>GSMTEIALIGNPNSGKTSLFNLITGHNQRVGNWPGVTVERKSGLVKKNKDLE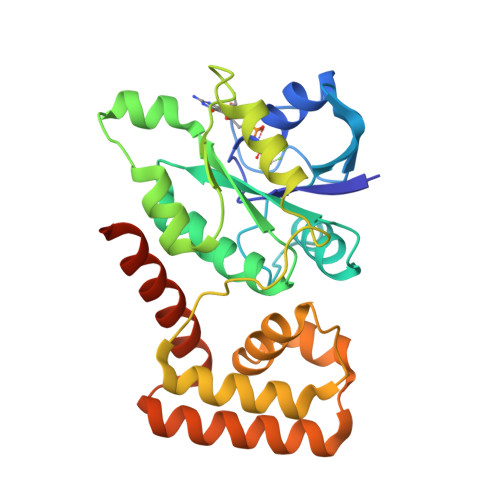IQDLPGIYSMSPYSPEEKVARDYLLSQRADSILNVVDATNLERNLYLTTQLIETGIPVTIALNMIDVLDGQGKKINVDKLSYHLGVPVVATSALKQTGVDQVVKKAAHTTTSTVGDLAFPIYDDRLEAAISQILEVLGNSVPQRSARFYAIKLFEQDSLVEAELDLSQFQRKEIEDIIRITEEIFTEDAESIVINERYAFIERVCQMAESHTEDFALTLS[2x]>[2x]MNWTVDIPIDQLPSLPPLPTDLRTRLDAALAKPAAQQPTWPADQALAMRTVLESVPPVTVPSEIVRLQEQLAQVAKGEAFLLQGGDCAETFMDNTEPHIRGNVRALLQMAVVLTYGASMPVVKVARIAGQYAKPRSA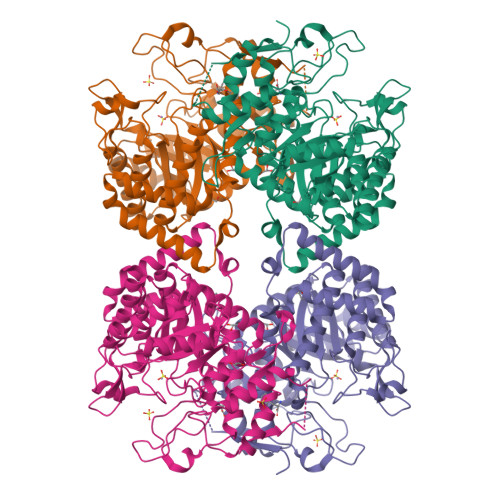DIDALGLRSYRGDMINGFAPDAAAREHDPSRLVRAYANASAAMNLVRALTSSGLASLHLVHDWNREFVRTSPAGARYEALATEIDRGLRFMSACGVADRNLQTAEIYASHEALVLDYERAMLRLSDGDDGEPQLFDLSAHTVWIGERTRQIDGAHIAFAQVIANPVGVKLGPNMTPELAVEYVERLDPHNKPGRLTLVSRMGNHKVRDLLPPIVEKVQATGHQVIWQCDPMHGNTHESSTGFKTRHFDRIVDEVQGFFEVHRALGTHPGGIHVEITGENVTECLGGAQDISETDLAGRYETACDPRLNTQQSLELAFLVAEMLRD> MGAQVSSQKVGAHENSNRAYGGSTINYTTINYYKDSASNAASKQDYSQDPSKFTEPLKDVLIKTAPALNSPNVEACGYSDRVLQLTIGNSTITTQEAANSVVAYGRWPEFIRDDEANPVDQPTEPDVATCRFYTLDTVMWGKESKGWWWKLPDALRDMGLFGQNMYYHYLGRSGYTVHVQCNASKFHQGALGVFAIPEYCLAGDSDKQRYTSYANANPGEKGGKFYSQFNRDTAVTSPKREFCPVDYLLGCGVL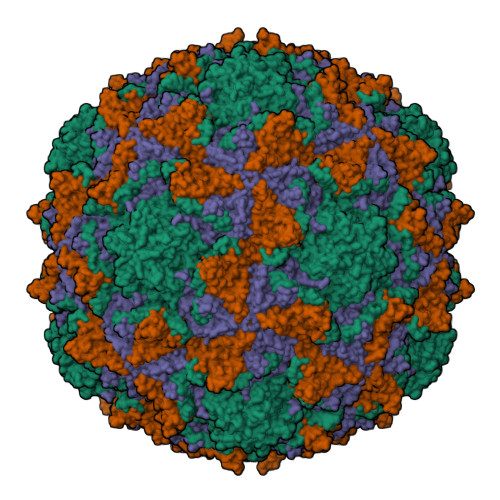LGNAFVYPHQIINLRTNNSATIVLPYVNAMAIDSMVKHNNWGIAILPLSPLDFAQESSVEIPITVTIAPMCSEFNGLRNVTAPKFQ;> GIEDLITEVAQGALTLSLPKQQDSLPDTKASGPAHSKEVPALTAVETGATNPLVPSDTVQTRHVIQRRSRSESTIESFFARGACVAIIEVDNEEPTTRAQKLFAMWRITYKDTVQLRRKLEFFTYSRFDMELTFVVTANFTNTNNGHALNQVYQIMYIPPGAPTPKSWDDYTWQTSSNPSIFYTYGAAPARISVPYVGLANAYSHFYDGFAKVPLKTDANDQIGDSLYSAMTVDDFGVLAIRVVNDHNPTKVTSKVRIYMKPKHVRVWCPRPPRAVPYYGPGVDYKDNLNPLSEKGLTTY;> GLPVLNTPGSNQYLTSDNYQSPCAIPEFDVTPPIDIPGEVKNMMELAEIDTMIPLNLENTKRNTMDMYRVTLSDSADLSQPILCFSLSPASDPRLSHTMLGEVLNYYTHWAGSLKFTFLFCGSMMATGKILVAYAPPGAQPPTSRKEAMLGTHVIWDLGLQSSCTMVVPWISNVTYRQTTQDSFTEGGYISMFYQTRIVVPLSTPKSMSMLGFVSACNDFSVRLLRDTTHISQSALPQ>MERELPIPVFLTEDEDSVHERMLSNFQDVSTLEGDFIYDATRPTAEQIAELKQLGLQNNLKIAFPQTSYGTYLEWLGECKGVFKNQPTKATGVITFTGVQGTIITKGTIVTTIATDEKQSIEFELLETKTIGENETVDIKAESRIVGTIGNVSKGSISVLLGSISGVKSITNKEDFRGGTDIEDEEHFRERVLVAEQEDKLSGASSDYIRWAKEVDGVGYAYVVSEWAGAGTVKVLILDKNRKAATQELIDKVQEYIYPLNISEGENRDGKAPIGALVTVVTPDTLLINVKASFIFSNGFSEETVLNNLKTKIDKYLDKIDLGGTVSYNAIQAIVGSMMLTDEGIEDFSNLTINDVKENIKLQDQVVGIGEIVNEVVG[12x];>[6x]MIASKKGKEMLLTLSPIYEQSIIMQSLYEAIGSEFDNLELLDEEIELQLFPQSATWGLGFWENRVGLITNLDEDMETRRRKVIAKLQSKYIMTPKRMSMILQSYTGANIKINENISPYTFGVELTSTQGFPKDLEDLYKRVNVIKPSHLAVSYKLVS;>MVIDIYLKNEKEKIDFHFPVNPQDSLSIKKEKRFETVDIVNLGEFDIKKEGEKIREISFKTFLPNLYDASYCRYSELKNPIEVVAMLEKWVDQAEPLRLIITGFGYNGLVTISSFSNTQTAGREEDRDIEITFRTYRELKIETLKKDTKSNTKTDLKDNRPNTQTKSKIYTVKASDTLYKIAKNLLGKGSRWPEIYNIPENKKVIGKNPNIIKKGQKLVIPSK[6x];>EEASFLNGSDVVILIDGVEELYMEEIKADFEQDEQSIKLLGCQNEISRVGTTKGSFSLNGYKTDSKFAKLGFRSFEIIYNLSNSETLGYESIRLKNCRLKKLPLINSKAGEIVKIEVEGSFRGYDLLNEL[6x];>[6x]EIPGFYNRFKAQAEKAAATGLKGRLAMPIRANWGDVGKVVTIKNDLRQLKNLFGDDMNYSAFKLGKLALLGNVKELLLYRLVDGNQKKGTLTLKDTTENSAKDVIKLETKYPTARNFNVTIKSNLVDSDKKDFIFFENTKQLFSSSIKGTIDEIVLEINSNLDNEYVIATKVADSDTILANVVNQALEGGNDGCTSITNESYLKALEEFERYSFDSFVLDGVADEALQETTKAWVAKNKELGKDILLFLGGKTEDNIKQINDKSKSFNDENIVNVGSSAYYENIKYTPSEVAVYIAALSVSKGITGSICNAKTIFEEVEPRLSQSEVKECLKSGTLVLDFDDGDVIIVDDVNTFKKYVDDKNEAMGYISNIMFINTINKDTSLKRKEFVGKIFNDATGQTTVICALKKYFEELMSQGIISEFNVDIDTELQATAKADEFYWKWDAVKVDVMKKIYGTGYL;>[6x]LDLKGSFLFDFEKGEFVKNADGTLKKCDKVQAYKQWCQKAILTPRYKKAAYTNIYGSEIKDLIASNLSQSAKELEITRLIKETILVHPYTKEVGEFSFNWLENSRLVEYEFDVLTIDDENIVIDG;>[3x]KIILNGKYDIANFNEGITLSEAIDGVAYKMDVSLVEPKQLKDINIKKGDKIILIDIAYESKKEETIFDGVVWETRRSEKSKKLTLSCRERTVYMEESEEQYQFKENTATQRIEYYCKQWNIPYYNLANTGKKLAKVIHKTNILDMIKKDLKETATKGGDLFRVRMDNKLKLFKLGTNANVYKLDSILEDANFTSSFNDAVTSVKVLGKSKDENTKAPIIGTYKKDADKFGTLQKIKQDEKIKNAKEAKKAAEAMFNSGEETISVDCAVDINRIRAGDKVSLKSKEYYVIDVTHTLDSRPKMKLNIGSLEYIRRKFY;>FNGIARILKENMNKSVANGTFGMGCELAEITANGLKVNGYKDEIQDYLVLENLTLKEDYFTFSDEALSGEYRHKHKIETPKELKPLRIGDNVLVAVMGAEFVVIGRVVNAKP[3x];>MREIAKKEMYHIDVVISAKGDGETKSKLSAMEKYMKQTEKRMQTLNRIKVNPAIKATDKASSVVNRVNNNMNKAKKTVTARIKATDNASPVANRASNNVNKAKKTVTARLKATDNASSTVNKVNNKIKEVAKPVPPVIIRGQDESSSIIDKVKAKIQNLKADTIIKIKSQADEAINTISRTKNKLQEFVSKRYEAAVKIRDEASSALRGLTGKIDSFVSGAISKFARLATTAGALIGGIGVGSAVKGFATFEQSMKNTQAVSGATGKEMEALTAKARQLGRETSFTAKDAGDAMYYMGMAGWKSEQMIKAIPDVLNLAAAGGTDLALTSDIVTDGLTALGMTANDTTEFVDVMAATITNSNTSVELMGETFKYVGSMGGALGVSMKDLSLATGLMASASVKGSMAGTSLRGGLVRLIKPPEEAASAIKKYGIELKKNKNGSLDLAGTIGSLREKLGGLKDVEKGVAISSIFGRTAMAGWAAVVNASESDFNKLTTAIAESEGEAKRIADMKLDTLSGQFEILKSAIDDVRISVGQRLGPMTRGFVEDLIKKMPQIGDAIVGVVEKFVNNFDKIKAGFQVLLPAIGSVIASVMVLKATFAFGGAIKSLSLLASTFGTAKLVAFGLTVGIGAIVIAFAGMTVAISNNKTAMMDLQTRFGSFGEYVTTIMETVGGVIKLTLGNLLIMLGGIGKGIGILLSDKSWDEKASSLKNLFGKTTAEIKTNTKEALSDINGETSNATALLKKSTSKELQGVTKAFSTAFDQSKNVTEKKSSDIARALTNGLKGLDDQSLTMMRGLNDNMAIILSGVTADMKPSDKVNKITKNLDDAFKAGKLSAQEYRSSIQETLNFISKYSADSSNNLKQGMSDAFNAFKEGTNIGGLKDGVTGMLNSLKATGPQALETLKGLGGKASEIFKGVDFNSSIDAQKTKVLQNLNSLGLEGTQAIDTLRTIFSQASSALDTTNLKQGLSNTFNSFKEGFNSGGIKNAINSMLGTINQAGPQMQQALGKMDGKMGQVFANVDFSTPIETQASKVLENLNNLGIEGPKALETVRSIFAQASSQIQGSASQTAQQANQEVANALTQGNPAVQQAGQQLGTDLTNGVVNGVQAGVPVVQQKSNELATATQNGVTNAVNSATPQIDNSNLTSGIDTAFNQATATVQQGASSMYNGAKQSFTQLAQIGREAGSSLYNGATTSFNMLATNVRVACSSMYNGARTSFTSLSSSAISAISAMCSSVVSQVSAMSSQIISYWNSVRATVSAPITASFNVKTTQTTVKRTVNESSGGILGNILDRFADGGVATRTSICGENGAEMVIPLTNTRRSRAIELYEQTGKMLGLGSTPSQKVGNSNIVNNVRQFPLANVLDTDNKEYKEATPNSVNSSNNTINLGGISINVQNSDNKEEMIQELLSQVESGIREALQDIG[3x]

Here, we reveal the extended and contracted atomic structures of an intact contractile-tailed phage (φCD508) that binds to and penetrates the protective S-layer of the Gram-positive human pathogen Clostridioides difficile. The virion can be divided into five distinct regions: the head, neck, tail, baseplate, and needle. Structures of purified φCD508 virions in both extended and contracted conformations were determined by single-particle EM of frozen-hydrated samples; the resolution ranged from 2.6 to 4.0 Å for the extended phage, and 2.9 to 4.2 Å for the contracted form.

Within the ring formed by the baseplate proteins lies the needle assembly; this is the other essential component presumed to be adapted for S-layer penetration. It is formed of two proteins, gp62 and gp63, providing a pointed end terminating the tail. Furthermore, exhaustive bioinformatics analysis of all proteins encoded within the φCD508 structural cassette (including those not modeled but identified by MS-MS analysis of purified virions) identified no enzymatic domains or motifs with predicted peptidoglycan hydrolase activity. It is also striking that the needle spike protein lacks the β-helix observed in other CIS structures, and instead, the OB-fold is connected directly to the metal-binding apex domain. The terminus of the φCD508 needle is an apex domain as reported in other phages; it displays a conserved hexahistidine motif coordinating a putative iron ion. However, the notable feature of φCD508 is that the needle lacks the otherwise widely conserved β-helix. It is currently unknown as to whether there is an advantage or requirement for this compact needle, but homology searches for other needle spikes lacking β-helix domains find widespread examples in phages infecting distantly related S-layer–producing bacteria. Peptidoglycan hydrolases that facilitate enzymatic penetration of the cell wall are a common feature of phage baseplates, including in the recent structure of a diffocin, a native C. difficile tailocin. It is striking that we find no obvious auxiliary domains with structural homology to peptidoglycan hydrolases in any of the φCD508 baseplate or needle proteins built to near completion within our cryoEM maps. Missing from the final structure are the tail fiber (gp67) and predicted receptor binding protein (gp68); only a short section of the tape measure protein (gp59) was modeled. Clear helical density with sidechain density is visible for the TMP lazo domain (dark blue). Interaction between the tape measure protein and the N-terminal bundle domain of the needle tip.>MLRVFILYAENVHTPDTDISDAYCSAVFAGVKKRTKVIKNSVNPVWNEGFEWDLKGIPLDQGSELHVVVKDHETMGRNRFLGEAKVPLREVLATPSLSASFNAPLLDTKKQPTGASLVLQVSYTPLPGAVPLFPPPTPLEPSPTLPDLDVVADTGGEEDTEDQGLTGDEAEPFLDQSGGPGAPTTPRKLPSRPPPHYPGIKRKRSAPTSRKLLSDKPQDFQIRVQVIEGRQLPGVNIKPVVKVTAAGQTKRTRIHKGNSPLFNETLFFNLFDSPGELFDEPIFITVVDSRSLRTDALLGEFRMDVGTIYREPRHAYLRKWLLLSDPDDFSAGARGYLKTSLCVLGPGDEAPLERKDPSEDKEDIESNLLRPTGVALRGAHFCLKVFRAEDLPQMDDAVMDNVKQIFGFESNKKNLVDPFVEVSFAGKMLCSKILEKTANPQWNQNITLPAMFPSMCEKMRIRIIDWDRLTHNDIVATTYLSMSKISAPGGEIEEEPAGAVKPSKASDLDDYLGFLPTFGPCYINLYGSPREFTGFPDPYTELNTGKGEGVAYRGRLLLSLETKLVEHSEQKVEDLPADDILRVEKYLRRRKYSLFAAFYSATMLQDVDDAIQFEVSIGNYGNKFDMTCLPLASTTQYSRAVFDGCHYYYLPWGNVKPVVVLSSYWEDISHRIETQNQLLGIADRLEAGLEQVHLALKAQCSTEDVDSLVAQLTDELIAGCSQPLGDIHETPSATHLDQYLYQLRTHHLSQITEAALALKLGHSELPAALEQAEDWLLRLRALAEEPQNSLPDIVIWMLQGDKRVAYQRVPAHQVLFSRRGANYCGKNCGKLQTIFLKYPMEKVPGARMPVQIRVKLWFGLSVDEKEFNQFAEGKLSVFAETYENETKLALVGNWGTTGLTYPKFSDVTGKIKLPKDSFRPSAGWTWAGDWFVCPEKTLLHDMDAGHLSFVEEVFENQTRLPGGQWIYMSDNYTDVNGEKVLPKDDIECPLGWKWEDEEWSTDLNRAVDEQGWEYSITIPPERKPKHWVPAEKMYYTHRRRRWVRLRRRDLSQMEALKRHRQAEAEGEGWEYASLFGWKFHLEYRKTDAFRRRRWRRRMEPLEKTGPAAVFALEGALGGVMDDKSEDSMSVSTLSFGVNRPTISCIFDYGNRYHLRCYMYQARDLAAMDKDSFSDPYAIVSFLHQSQKTVVVKNTLNPTWDQTLIFYEIEIFGEPATVAEQPPSIVVELYDHDTYGADEFMGRCICQPSLERMPRLAWFPLTRGSQPSGELLASFELIQREKPAIHHIPGFEVQETSRILDESEDTDLPYPPPQREANIYMVPQNIKPALQRTAIEILAWGLRNMKSYQLANISSPSLVVECGGQTVQSCVIRNLRKNPNFDICTLFMEVMLPREELYCP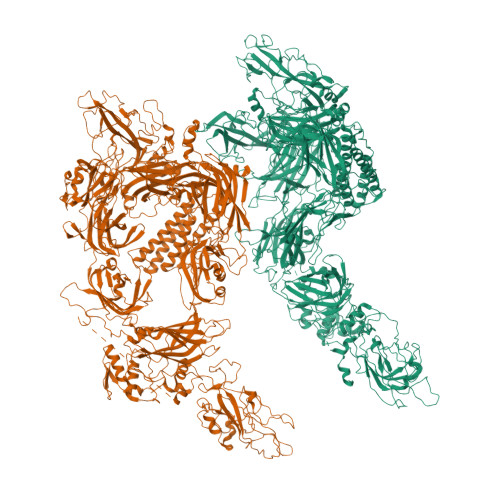PITVKVIDNRQFGRRPVVGQCTIRSLESFLCDPYSAESPSPQGGPDDVSLLSPGEDVLIDIDDKEPLIPIQEEEFIDWWSKFFASIGEREKCGSYLEKDFDTLKVYDTQLENVEAFEGLSDFCNTFKLYRGKTQEETEDPSVIGEFKGLFKIYPLPEDPAIPMPPRQFHQLAAQGPQECLVRIYIVRAFGLQPKDPNGKCDPYIKISIGKKSVSDQDNYIPCTLEPVFGKMFELTCTLPLEKDLKITLYDYDLLSKDEKIGETVVDLENRLLSKFGARCGLPQTYCVSGPNQWRDQLRPSQLLHLFCQQHRVKAPVYRTDRVMFQDKEYSIEEIEAGRIPNPHLGPVEERLALHVLQQQGLVPEHVESRPLYSPLQPDIEQGKLQMWVDLFPKALGRPGPPFNITPRRARRFFLRCIIWNTRDVILDDLSLTGEKMSDIYVKGWMIGFEEHKQKTDVHYRSLGGEGNFNWRFIFPFDYLPAEQVCTIAKKDAFWRLDKTESKIPARVVFQIWDNDKFSFDDFLGSLQLDLNRMPKPAKTAKKCSLDQLDDAFHPEWFVSLFEQKTVKGWWPCVAEEGEKKILAGKLEMTLEIVAESEHEERPAGQGRDEPNMNPKLEDPRRPDTSFLWFTSPYKTMKFILWRRFRWAIILFIILFILLLFLAIFIYAFPNYAAMKLVKPFS[2x]> AMIIANADGCTPYEVARGVTIVRGEGAYVYDAEGRGLIDLSNSFGSVMLGHQDPVVTEAVLKTVRSGVPAAASLDLQNHLAEQIAGDLPGDQRVAFFKTGTAATRAAASAARQVTGKRLIASCGYHGYDLMWEFTPPGQPNSEDVLHCYHLPELIDQVLDKHAHELAAVIIAPDYIHVSPEYIADLFERCERVGVVTIADEVKHGYRLRQGASVTEASVVADMYTYAKGISNGWPLSCVAGDERFLKPLAEFVSTLTFEAPSFAAASATLDRLAELDVQAQLAIDGARFVSEAAKMISTRDLPIEMAGTGAAFQFVCAEEVEEVLLPHALAEGLILEPSDQQYPSACFRGEVVDDALERLDRALTTMAAARPDLVGREVTQLDRVNAAFCQMDGLPGRPDGWSLDQCVEYVTAQL

GenB2 acts as an isomerase, converting C2a into C2 by changing the stereochemistry of the chiral center C-6′. Four genes encoding PLP-dependent enzymes (GenB1–GenB4) identified in the gentamicin BGC and a methyltransferase, GenL, from outside the BGC, are responsible for the last steps of gentamicin C complex biosynthesis. The structure of GenB2 shows, as expected, a characteristic PLP-dependent enzyme class I fold. Similar to other enzymes from this family, the active site of GenB2 is located in a deep cavity formed by a groove in the interface between the two protomers of the dimer, and each subunit contributes with essential residues for the substrate and cofactor binding.

GenB2 was successfully produced, and the enzyme purified close to homogeneity showed a pink color, indicating copurification with the coenzyme. Although we have made several attempts to obtain the GenB2 structure in the resting complex (internal aldimine), we did not observe the formation of the Schiff base between the coenzyme and Lys227 in any of the tested crystal and solved structures. Based on that, we assumed that pyridoxamine 5-phosphate (PMP) is the predominant coenzyme state bound to the enzyme. Each dimer of GenB2 has two PMP molecules bound at the interfaces between the protomers. Residues of both protein molecules are responsible for anchoring the coenzyme in the binding site. The PMP molecule forms an extensive hydrogen bond network with protein residues. These residues include the critical catalytic residue Lys227, which interacts with the primary amine of the coenzyme, and the conserved (in type I PLP-dependent proteins) Asp199, which interacts with the nitrogen of the pyridine ring of PMP. Further interactions include an interaction of the main chain NH of Tyr124 with the pyridine nitrogen of PMP (all of these from the same protomer, here called A). Tyr124 also performs an edge-π interaction with the PMP ring. Additionally, when we superpose the structure of holo GenB2 with holo GenB2 in complex with G418, we can observe that the substrate does not cause any significant conformation changes in the region of the substrate binding site.>THLFEGVGVALTTPFTNNKVNLEALKAHVNFLLENNAQAIIVNGTTAESPTLTTDEKELILKTVIDLVDKRVPVIAGTGTNDTEKSIQASIQAKALGADAIMLITPYYNKTNQRGLVKHFEAIADAVKLPVVLYNVPSRTNMTIEPETVEILSQHPYIVALKDATNDFEYLEEVKKRIDTNSFALYSGNDDNVVEYYQRGGQGVISVIANVIPKEFQALYDAQQSGLDIQDQFKPIGTLLSALSVDINPIPIKALTSYLGFGNYELRLPLVSLEDTDTKVLREAYDTF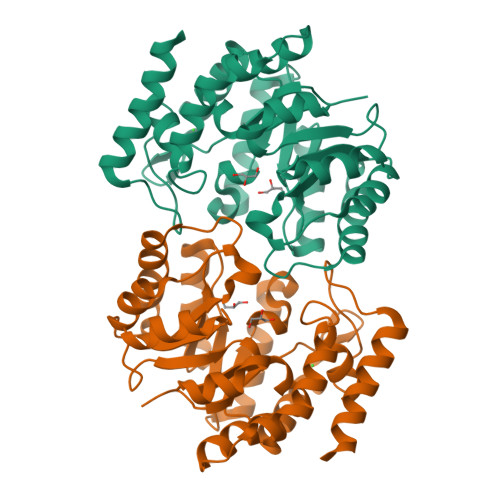KAGE[4x]> GMAYTTTVKLDGDTKTYTLSPTVKKYTLMDLGFVKGRSGAFSFERSLDPTSPYQAAFKLKMTVNADLTGFKMTTV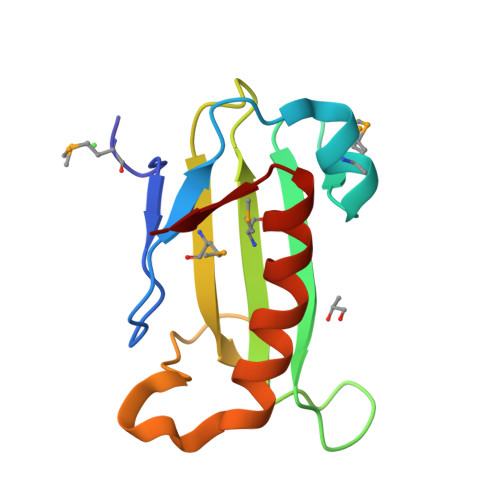TGNGVQRANIFKNDAHPEAVEQLRYILANFIERDILTTD> QYAPQTQSGRTSIVHLFEWRWVDIALECERYLGPKGFGGVQVSPPNENIVVTNPSRPWWERYQPVSYKLCTRSGNENEFRDMVTRCNNVGVRI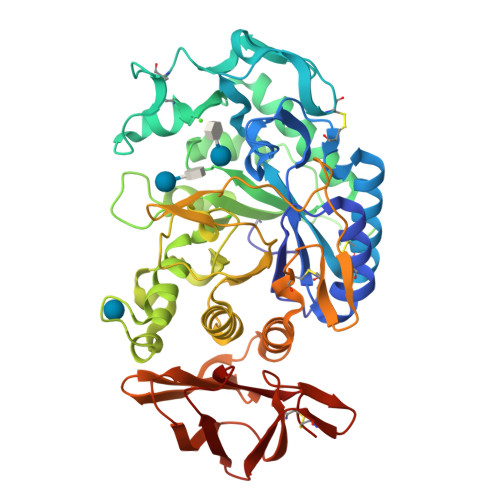YVDAVINHMCGSGAAAGTGTTCGSYCNPGSREFPAVPYSAWDFNDGKCKTASGGIESYNDPYQVRDCQLVGLLDLALEKDYVRSMIADYLNKLIDIGVAGFRIDASKHMWPGDIKAVLDKLHNLNTNWFPAGSRPFIFQEVIDLGGEAIQSSEYFGNGRVTEFKYGAKLGTVVRKWSGEKMSYLKNWGEGWGFMPSDRALVFVDNHDNQRGHGAGGASILTFWDARLYKVAVGFMLAHPYGFTRVMSSYRWARNFVNGEDVNDWIGPPNNNGVIKEVTINADTTCGNDWVCEHRWREIRNMVWFRNVVDGEPFANWWDNGSNQVAFGRGNRGFIVFNNDDWQLSSTLQTGLPGGTYCDVISGDKVGNSCTGIKVYVSSDGTAQFSISNSAEDPFIAIHAESKL>MSLRIRVPATTANLGPGFDSCGLALTLYLTLDIGAEADSWYIEHNIGGGIPHDETNVIIETALNLAPNLTPHHLVMTCDIPPARGLGSSSAAVVAGIELANTLAELNLSKEEKVRIAAEIEGHPDNVAPAVLGNWVVGAKLDGEDFYVRHLFPDCALIAFIPKAELLTSESRGVLPDTLPFKEAVQASSIANVMIAAILRNDMTLAGEMMERDLWHEKYRSQLVPHLAQIRDVAKNQGAYAACLSGAGPTVLVFAPRNLANKLQTSLQTLEIDADVLLLDVEGSGAEVFREGH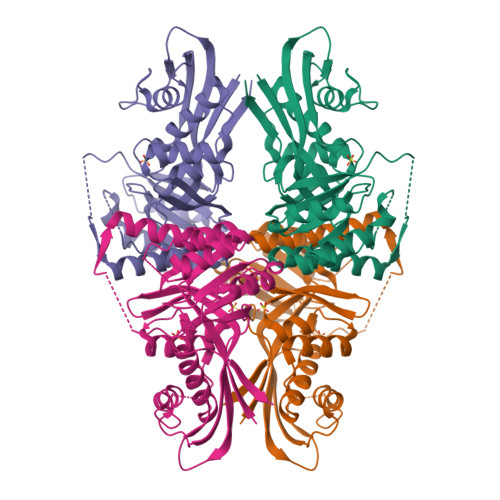HHHHH[2x]> TLQQDRSPDVINIHSLDEYHNIVSENILTVLWFWASDCGPCKE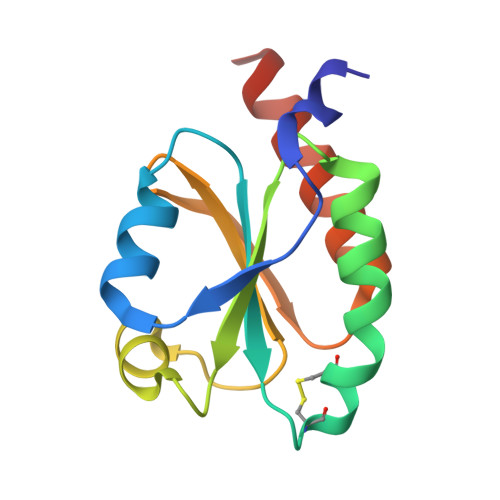IEEPLKKMAEDFPNVVFAKVNAEENQKIVEKLNVKSLPTAIIAKGGKYLGHVVGADPDRLREKVQNIIANLEHHHHHH> V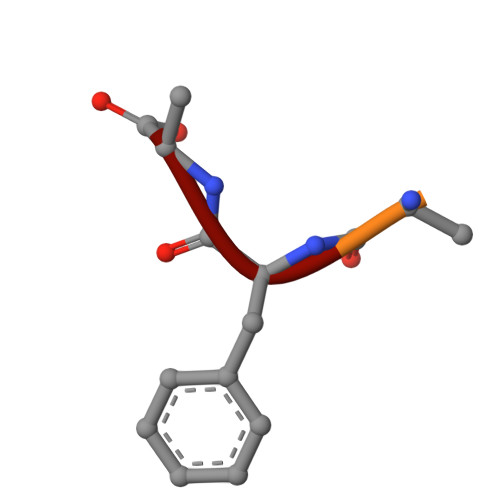TSFA(3R)-3-azanyl-4-oxidanylidene-4-[[3-(trifluoromethyloxy)phenyl]amino]butanoic acid | C11 H11 F3 N2 O4 | 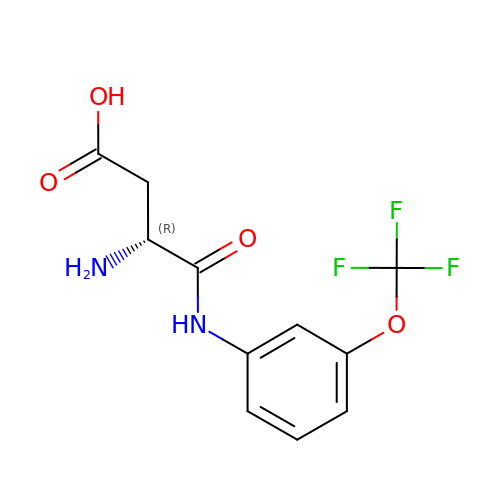LHAPJSHUQJWWEP-MRVPVSSYSA-N1,3-DIPHENYLUREA | C13 H12 N2 O | 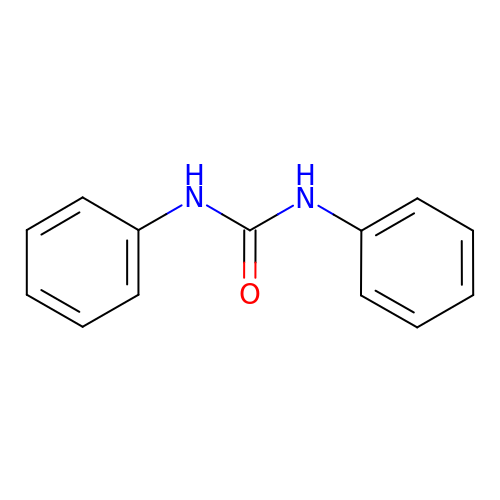GWEHVDNNLFDJLR-UHFFFAOYSA-N> MTEFDEIVKPDDKEETSESTEENLESTEETSESTEESTEESTEESTEDKTVETIEEENENKLEPTTTDEDSSKFDPVVLEQRIASLEQQVTTFLSSQMQQPQQVQQTQSDVTESNKEDNDYSDEE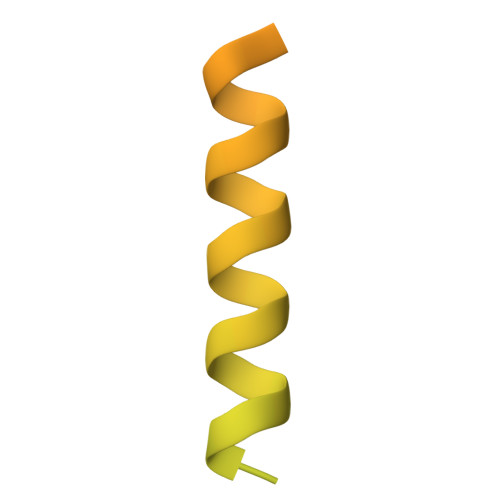LVDKLDLD>MAKVYKDLREFLEVLEQEGQLIRVKEEVNPEPDIAAAGRAAANLGKNQPAVFFEKIKGYKYSVVTNVHGSWQNHALMLGLDKNTSTKDQFYELNRRWDKFPVPPNVVKREAAPCKENVIDKDINLFEILPLYRINEQDGGFYISKASVVTADPEYPDDFNKLNVGTYRIQVKDRDRVGIQALAMHDIAVQLEKAEAENKPLPIAITIGNNPLVTFMASTPVGYNQNEYEFVGALQD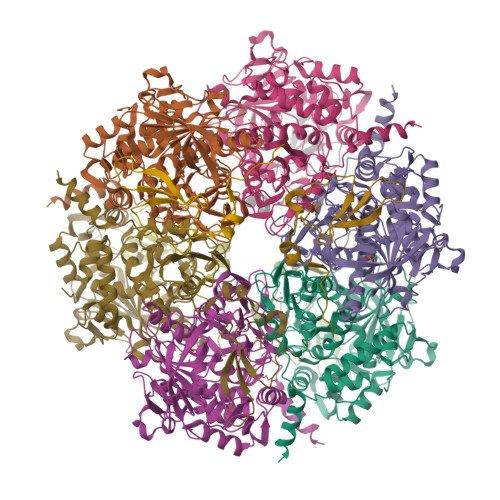GVPMDIVKSDLYDHLYVPAGSEVVLEGHIIPRVRTVEGPFGEFPGSYSGARLQCEVKIDRITHRTNPIFENLYLGIPWTEIDYLMALNTSVPLYKQLKETMPEVVAVNAMYTHGIGVIISTKVRYGGYAKGVAFRLLSTPHGMPYSKIVIVVDEFVDPFNLEQVMWALTTRVHPGKDVSIIENCPGMPLDPSTNPPGMHTKMIIDATTPVPPEPNPRETQLLDPPDGTEEWEEKLKELLKNQNR[6x];>MKCHRCGSDNVRKMVDSPVGDAWEVYVCEKCCYSWRSTENPVVMEKFKLDDNKIANMGVIPPIPPLKK[6x]>AYTTFSQTKNDQLKEPMFFGQPVNVARYDQQKYDIFEKLIEKQLSFFWRPEEVDVSRDRIDYQALPEHEKHIFISNLKYQTLLDSIQGRSPNVALLPLISIPELETWVETWAFSETIHSRSHTHIIRNIVNDPSVVFDDIVTNEQIQKRAEGISSYYDELIEMTSYWHLLGEGTHTVNG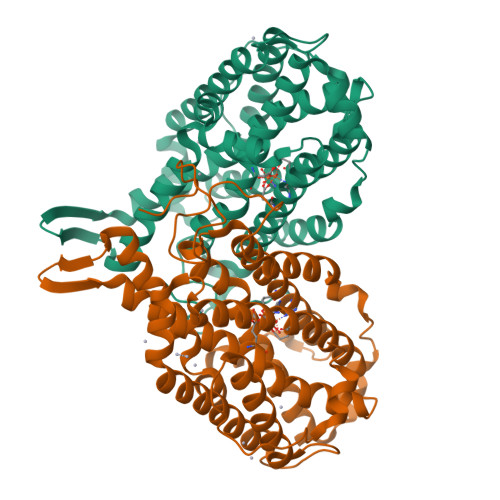KTVTVSLRELKKKLYLCLMSVNALEAIRFYVSFACSFAFAERELMEGNAKIIRLIARDEALHLTGTQHMLNLLRSGADDPEMAEIAEECKQECYDLFVQAAQQEKDWADYLFRDGSMIGLNKDILCQYVEYITNIRMQAVGLDLPFQTRSNPIPWINTWLVSDNVQVAPQEVEVSSYLVGQIDSEVDTDDLSNFQL[2x]>MPKPYVAINMAELKNEPKTFEMFASVGPKVCMVTARHPGFVGFQNHWQIGILPFGNRYGGAKMDMTKESSTVRVLQYTFWKDWKDHEEMHRQNWSYLFRLCYSCASQMIWGPWEPIYEIIYANMPINTEMTDFTAVVGKKFAEGKPLDIPVISQPYGKRVVAFAEHSVIPGKEKQFEDAIVRTLEMLKKAPGFLGAMVLKEIGVSGIGSMQFGAKGFHQVLENPGSLEPDPNNVMYSVPEAKNTPQQYIVHVEWANTDALM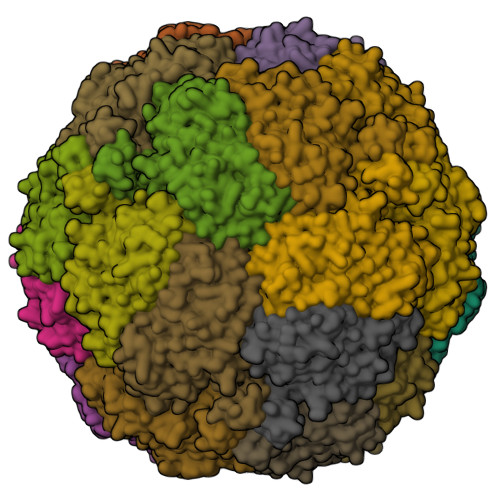FGMGRVLLYPELRQVHDEVLDTLVYGPYIRILNPMMEGTFWREYLNENAWRHPQFGG[4x]> MGHHHHHHAMEGKITPVSVKKVDDKVTLYKTTATADSDKFKISQILTFNFIKDKSYDKDTLVLKATGNINSGFVKPNPNDYDFSKLYWGAKYNVSISSQSNDSVNVVDYAPKNQNEEFQVQNTLGYTFGGDISISNGLSGGLNGNTAFSETINYKQESYRTTLSRNTNYKNVGWGVEAHKIMNNGWGPYGRDSFHPTYGN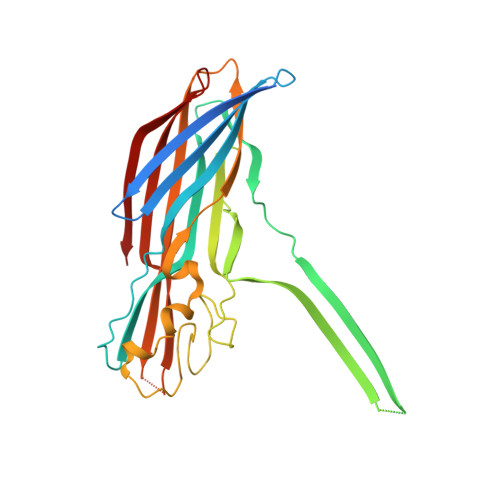ELFLAGRQSSAYAGQNFIAQHQMPLLSRSNFNPEFLSVLSHRQDGAKKSKITVTYQREMDLYQIRWNGFYWAGANYKNFKTRTFKSTYEIDWENHKVKLLDTKETENNK>[2x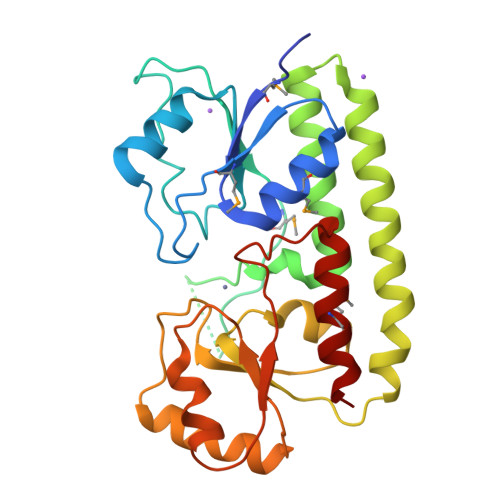]GQKESQTGKGMKIVTSFYPIYAMVKEVSGDLNDVRMIQSSSGIHSFEPSANDIAAIYDADVFVYHSHTLESWAGSLDPNLKKSKVKVLEASEGMTLERVPGLEDVEAGDGVDEKTLYDPHTWLDPEKAGEEAQIIADKLSEVDSEHKETYQKNAQAFIKKAQELTKKFQPKFEKATQKTFVTQHTAFSYLAKRFGLNQLGIAGISPEQEPSPRQLTEIQEFVKTYKVKTIFTESNASSKVAETLVKSTGVGLKTLNPLESDPQNDKTYLENLEENMSILAEELK>MGLSLPKEKGLILCLWSKFCRWFQRRESWAQSRDEQNLLQQKRIW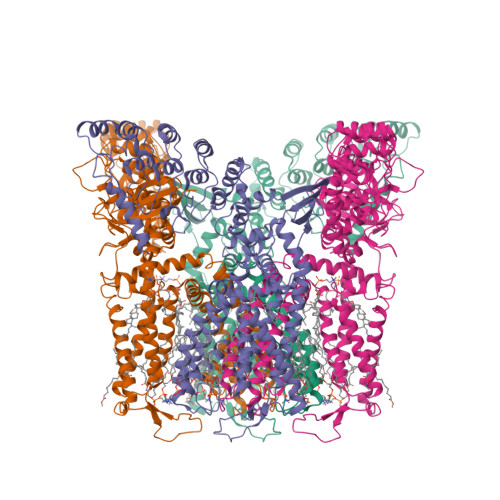ESPLLLAAKDNDVQALNKLLKYEDCKVHQRGAMGETALHIAALYDNLEAAMVLMEAAPELVFEPMTSELYEGQTALHIAVVNQNMNLVRALLARRASVSARATGTAFRRSPCNLIYFGEHPLSFAACVNSEEIVRLLIEHGADIRAQDSLGNTVLHILILQPNKTFACQMYNLLLSYDRHGDHLQPLDLVPNHQGLTPFKLAGVEGNTVMFQHLMQKRKHTQWTYGPLTSTLYDLTEIDSSGDEQSLLELIITTKKREARQILDQTPVKELVSLKWKRYGRPYFCMLGAIYLLYIICFTMCCIYRPLKPRTNNRTSPRDNTLLQQKLLQEAYMTPKDDIRLVGELVTVIGAIIILLVEVPDIFRMGVTRFFGQTILGGPFHVLIITYAFMVLVTMVMRLISASGEVVPMSFALVLGWCNVMYFARGFQMLGPFTIMIQKMIFGDLMRFCWLMAVVILGFASAFYIIFQTEDPEELGHFYDYPMALFSTFELFLTIIDGPANYNVDLPFMYSITYAAFAIIATLLMLNLLIAMMGDTHWRVAHERDELWRAQIVATTVMLERKLPRCLWPRSGICGREYGLGDRWFLRVEDRQDLNRQRIQRYAQAFHTRGSEDLDKDSVEKLVPRGSAAAWSHPQFEK[4x]>[2x]MAEQVKPAGVKPKGTVPPPKGNAPAPKANGAPGGASVIKEQDAAKMRRFLFQRTETRSTKWYQIFDTEKLDDEQVVGGHLALLGVLGFIMGIYYISGIQVFPWGAPGFHDNWFYLTIKPRMVSLGIDTYSTKTADLEAAGARLLGWAAFHFLVGSVLIFGGWRHWTHNLTNPFTGRCGNFRDFRFLGKFGDVVFNGTSAKSYKEALGPHAVYMSLLFLGWGIVMWAILGFAPIPDFQTINSETFMSFVFAVIFFALGIYWWNNPPNAAIHLNDDMKAAFSVHLTAIGYINIALGCIAFVAFQQPSFAPYYKELDKLVFYLYGEPFNRVSFNFVEQGGKVISGAKEFADFPAYAILPKSGEAFGMARVVT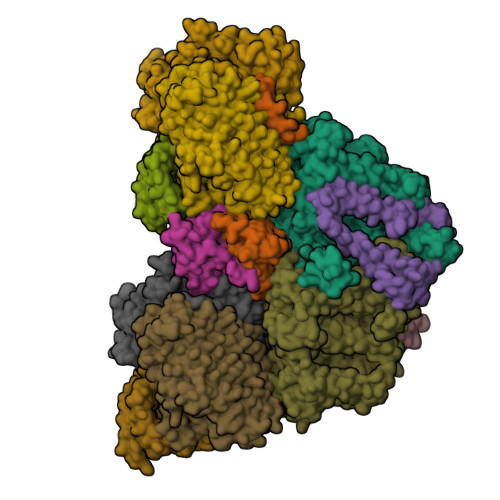NLIVFNHIICGVLYVFAGVYHGGQYLLKIQLNGMYNQIKSIWITKGRDQEVQVKILGTVMALCFATMLSVYAVIVWNTICELNIFGTNITMSFYWLKPLPIFQWMFADPSINDWVMAHVITAGSLFSLIALVRIAFFAHTSPLWDDLGLKKNSYSFPCLGPVYGGTCGVSIQDQLWFAMLWGIKGLSAVCWYIDGAWIASMMYGVPAADAKAWDSIAHLHHHYTSGIFYYFWTETVTIFSSSHLSTILMIGHLVWFISFAVWFEDRGSRLEGADIQTRTIRWLGKKFLNRDVNFRFPVLTISDSKLAGTFLYFGGTFMLVFLFLANGFYQTNSPLPPPVSHAAVSGQQMLAQLVDTLMKMIA;> MAEPVENKNQAPAPGAKVPPKGAPAAPKAGAPAAPKGPVAPKAGAPAAKTGASAAKQAGKPRLASLGVTLGRSGVRQESALPYVKPKAVPPPKPAAPAAKGAPAPKGAPAAPAAKAAPGAPVAKAAPKAKKHYFIIENLCVGCGLCLDKCPPKVNAIGYKFYGDVQEGGFRCYIDQAACISCSACFSGDECPSGALIEVLPDGEVLDFSYTPPERLDFDLRFLHRFHREAR;>MDKNSNGKLIALAVGGAVLMGALFFSVSFLTGYIPAPNHSAILTPLRSFMGWFLLIFCASIIIMGLGKMSSAISDKWFLSFPLSIFVIVMVMFLSLRVYWEKGRTTTVDGKYIRTTAELKEFLNKPAATSDVPPAPAGFDFDAAKKLVDVRCNKCHTLDSVADLFRTKYKKTGQVNLIVKRMQGFPGSGISDDDAKTIGIWLHEKF[2x];> MQPQLSRPQTASNQVRKAVSGPWSGNAVHKAEKYFITSAKRDRDGKLQIELVPASGRRKLSPTPEMIRRLIDGEIEIYILTTQPDIAIDMNKEIIDMENRYVIDFDKRGVKWTMREIPVFYHEGKGLCVELHNKIYTLDQFFK;> MDAKTTILEVLKKEGKPMSAGQIAEKSGLERKEVDKAMKSLKEEELIVSPKRCYWTPKV;> MDIRRLILAFILPPAAVMNKEAGTIMLTGILTLWGWIPGVVAALIMISKEQSGKTAEA;>MALFGSNDVTTAHSDYEIVLEGGSSSWGKVKARAKVNAPPASPLLPADCDVKLNVKPLDPAKGFVRISAVFESIVDSTKNKLTIEADIANETKERRISVGEGMVSVGDFSHTFSFEGSVVNLFYYRSDAVRRNVPNPIYMQGRQFHDILMKVPLDNNDLIDTWEGTVKAIGSTGAFNDWIRDFWFIGPAFTALNEGGQRISRIEVNGLNTESGPKGPVGVSRWRFSHGGSGMVDSISRWAELFPSDKLNRPAQVEAGFRSDSQGIEVKVDGEFPGVSVDAGGGLRRILNHPLIPLVHHGMVGKFNNFNVDAQLKVVLPKGYKIRYAAPQYRSQNLEEYRWSGGAYARWVEHVCKGGVGQFEILYAQ[6x]> MNQQGFVISNELRQQQSELTSTWDLMLQTRINLARSAARMMMDASNQQSSAKTDLLQNAKTTLAQA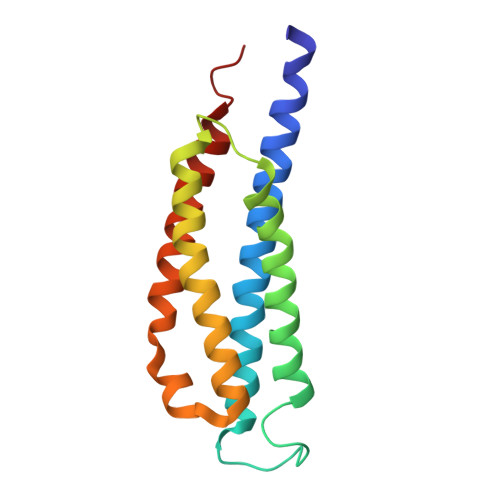AAHYANFKNMTPLPAMAEASANVDEKYQRYQAALAELIQFLDNGNMDAYFAQPTQGMQNALGEALGNYARVSENLYRQTF>[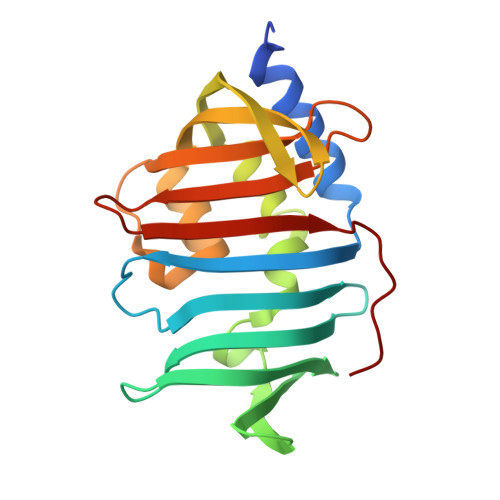2x]MHHHHHHGPLPDAKPLVEEATAQTKALKSAHMVLTVNGKIPGLSLKTLSGDLTTNPTAATGNVKLTLGGSDIDADFVVFDGILYATLTPNQWSDFGPAADIYDPAQVLNPDTGLANVLANFADAKAEGRDTINGQNTIRISGKVSAQAVNQIAPPFNATQPVPATVWIQETGDHQLAQAQLDRGSGNSVQMTLSKWGEKVQVT>MGKIVEIHPTTRHEGHTKLVLKVDDEGIVEKGAYLSVTPVRGFEKFLVGKPAEFAPIAVSRFCGICPVAHATSAVEAIEDACDITPPKDGLLLRELCGIGNKMHSHPLHQFLISPDYVPKDDSNEFIKRVQAMRRIGQYIVDAVGGEAIHSPNIKVGGMAKQITESTKAKMYYKCKEYEKLAKEQLEYLIPIFESRTLNDGTELPEKLGYHDFGYIATHPTYGDRTKIDQDKVVEYTPFDVYDKDVAIQSSTTVPTYNGRLMEVGPRARFSKFFDFKEKGAMALHIARAYEISVLVKRAMEILDELNVNGKTMSDEPIVGDGEKLGLGVHEAARGHNTHQAVIDKDGNIVYYNAIVATTWNIPVISKAVEGTHYKFAEHIVRAYDPCISCATHMIIKDYDDKIIGEKILK[4x];>MDPFGKYKTVVSARAADKTILKKCQDGGIVSAAYIYGLENGLLDGVIVADKDDKLQTTPKVATTVDEVLEAAGTKYTVCPTISVIKSAVREYGCEKLGVVGTPCQIIATRKLMKYPIGFRHVPDKLALIVGIFCMENFPYNGMKTIIEEHCGIKMEDVAKTDIGKGKFWVYSKWGDVKSIKLKETHPYEQQSCHVCMDYTAELADISTGSVGSPDGWSTVFIRTAQGEEFFNKMVEAGALEVKPIEEVKPGLGLVEKLSLTKKEKNAKEIEHRKEIGLPVPY[4x];>MVKIAHIHLCGCTGCLISLADTYEQLLDILNSVELVYALTLVDEKTEIRETDDKILIEREIPDDIDIALVEGSVCLEDEHSMKDVFDARRKSKIVVALGACAATGGITRFCRGGQMSKPVHSSFVPIGDLIKVDLALPGCPPSPEALVNLITAALNGDTEYLEIYAELAKKTEACGCDLLVNVINKSLCMGCGSCAASCPTRAIEMIDGKPNVLKELCIKCGACSLQCPRIRFPKLIEEIE[4x]

FRHs catalyze the reversible H2 oxidation coupled to the reduction of coenzyme F420 (8‐hydroxy‐5‐deazaflavin, ΔG°′ = −10 kJ mol−1). The overall reaction requires three components: the large subunit (FRHA) that harbors the [NiFe] center and oxidizes H2, and the small subunit (FRHG), which contains three [4Fe–4S] clusters to transfer electrons to the flavin adenine dinucleotide (FAD) located in the F420‐reducing module (FRHB, harboring an additional [4Fe–4S] cluster). FRHABG dimerizes and forms dodecameric assemblies of about 16 nm in diameter with a spherical shape and a hollow core. Here, by characterizing the native hydrogenase from the marine methanogen Methanothermococcus thermolithotrophicus (belonging to the Methanococcales order), we provided an unprecedented functional understanding of this enzyme via a synergistic approach of biochemistry, X‐ray crystallography, and spectroscopy.

Despite its sequence conservation with the two other structural homologs, we found that the [NiFe]‐containing FRH from M. thermolithotrophicus (MtFRH) exhibits a dynamic equilibrium between a dodecameric and dimeric state in solution, as highlighted by size exclusion chromatography and native polyacrylamide gel electrophoresis (PAGE). It was therefore not surprising to observe several crystalline forms containing either a dodecameric cubic organization (MtFRHcube) or only a single FRH dimer (MtFRHdimer1 −3). Based on the four X‐ray crystallographic structures obtained, we confirmed that MtFRH shares the basic organization previously observed with an elementary dimer of FRHABG heterotrimers that further builds into a dodecameric unit. Surface analyses through bioinformatics confirmed that the dodecameric state might be less stable in solution based on the structure of M. barkeri (MbFRH). However, considering the molecular crowding effect and the naturally high FRH expression (≈1% of total cytoplasmic protein), we propose that MtFRH forms a dodecamer of ≈1.2 MDa in vivo. The dodecameric assembly has been hypothesized to provide stability, protect redox centers, or keep the metal clusters at optimal distances. Nevertheless, the comparison of Fe‐containing MtFRHdimer2 and Fe‐depleted MtFRHcube does not reveal any structural rearrangement of the surrounding residues or the ones in the vicinity of the [NiFe] site. Therefore, the importance of the additional Fe site in modulating the redox properties of the [NiFe] center remains to be experimentally investigated.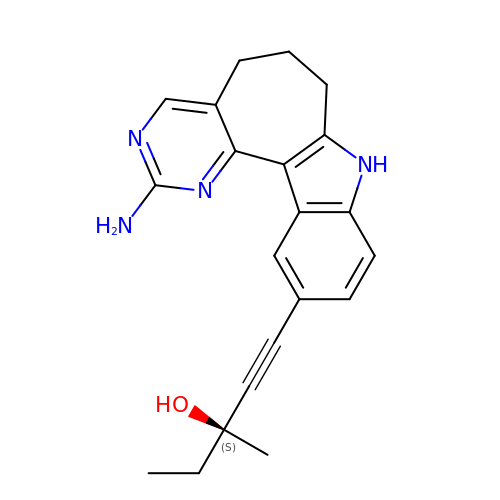(3~{S})-1-(4-azanyl-3,5,12-triazatetracyclo[9.7.0.0^{2,7}.0^{13,18}]octadeca-1(11),2,4,6,13(18),14,16-heptaen-16-yl)-3-methyl-pent-1-yn-3-ol | C21 H22 N4 O | ALQLTPNCVCECNJ-NRFANRHFSA-N> KPFANTKKTLENQVEELTEKCSLKTDEFLKAKEKINEIFEKLNTIRDEVIKKKNQNEYYR;> DVSQKIKDIDDQIQQLLLKQRHLLSKMASSMKSLKNCQKELISTQILQFEAQNMDVSMNDVIGFFNEREADLK;> MALNDNPIPKSVPLHPKSGKYFHNLHARDLSNIYQQCYKQIDETINQLVDSTSPSTIGIEEQVADITSTYKLLSTYESESNSFDEHIKDLKKNFKQSSDACPQIDLSTWDKYRTGELTAPKLSELYLNMPTPEPATMVNNTDTLKILKVLPYIWNDPTCVIPDLQNPADEDDLQIEGGKIELTCPITCKPYEAPLISRKCNHVFDRDGIQNYLQGYTTRDCPQAACSQVVSMRDFVRDP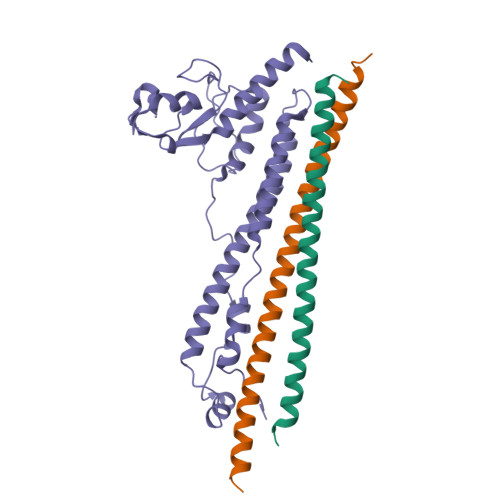IMELRCKIAKMKESQEQDKRSSQAIDVL>GEEDKTNYGSRTVLVYIAGDNSLSRFASEDLNEMIEGMQSVDDNHNNLLVYMDKGSNPKLIRLRKDKDVVVQDVIATYDAQNSVDVDVMKNVFTTAFSHYPADSYGVVFWSHGDGWLPYNNPSTRWWGQDTGNGDNRMNIPDLNEALSVAPHFDFILFDACYMQSVEVVYQLRNRADYFIGSPTEIPGPGAPYEVVVPALFAVNSPAVSIAENYYSVYAKKYNSTGAGISNENWTGGVSISVIKSSELSALAAATRDVLQTAVSMQQSHNIDISSILCYDPLRENNYHDLMGLMQSIQGNSQAFNHYKEMYKNAVIWKNTTDNNYCTYSSGYGKMVSMDGFEGVSTYILRENNSSQEKYYRQFV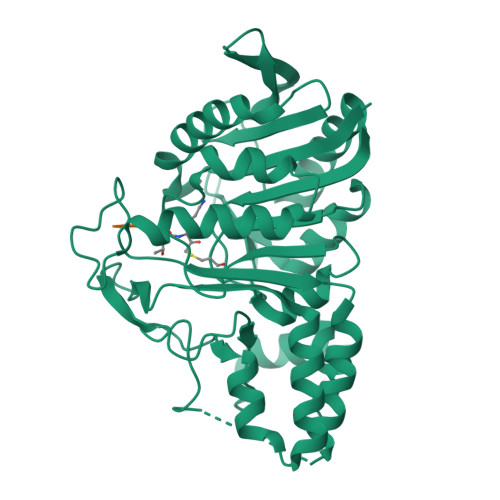EWYSAADWDSVDW[2x]N-[(2-fluorophenyl)methyl]-1H-pyrazol-4-amine | C10 H10 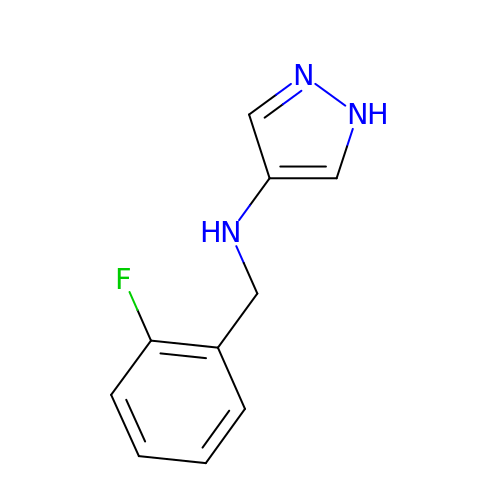F N3 | PDSIYANAENEXNZ-UHFFFAOYSA-N>[3x]GCTGG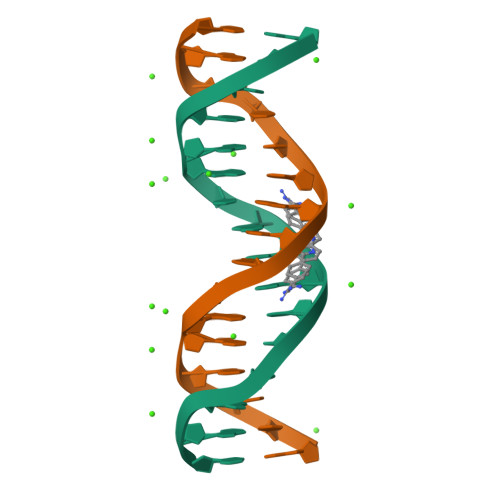ATATATCCAGC> MAVLGLQGVRGGVGTTTITAALAWSLQMLGENVLVVDACPDNLLRLSFNVDFTHRQGWARAMLDGQDWRDAGLRYTSQLDLLPFGQLSIEEQENPQHWQTRLSDICSGLQQLKASGRYQWILIDLPRDASQITHQLLSLCDHSLAIVNVDANCHIRLHQQALPDGAHILINNFRIGSQVQDDIYQLWLQSQR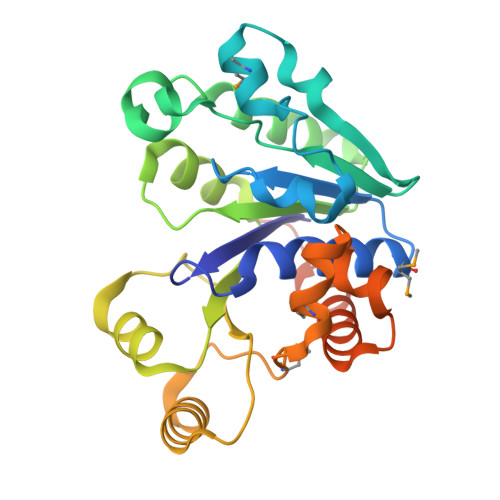RLLPMLIHRDEAMAECLAAKQPVGEYRSDALAAEEILTLANWCLLNYSGLKTPVGSKSAAALEHHHHHH>[2x]GKPVVAIVGRPNVGKSTIFNRIAG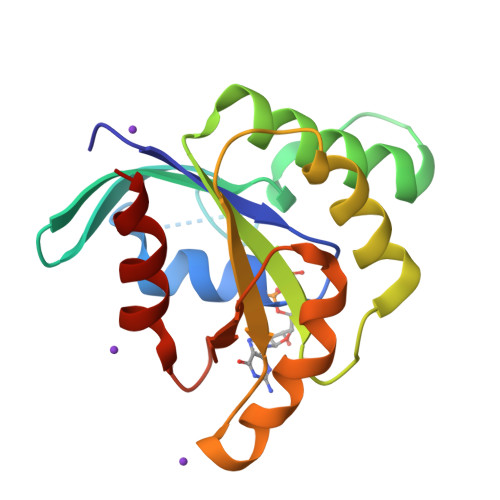ERISIVEDTPGVTRDRIYSSAEWLNYDFNLIDTGGIDIGDEPFLAQIRQQAEIAMDEADVIIFMVNGREGVTAADEEVAKILYRTKKPVVLAVNKLDNTEMRANIYDFYSLGFGEPYPISGTHGLGLGDLLDAVAEHF>[6x]GSQDSTSDLIPAPPLSKVPLQQNFQDNQFQGKWYVVGLAGNAILREDKDPQKMYATIYELKEDKSYNVTSVLFRKKKCDYWI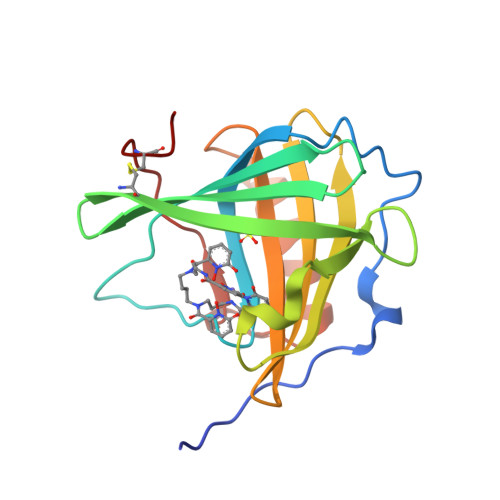RTFVPGSQPGEFTLGNIKSYPGLTSYLVRVVSTNYNQHAMVFFKKVSQNREYFKITLYGRTKELTSELKENFIRFSKSLGLPENHIVFPVPIDQCIDG> MSETQSQTMTRPQDLSLSDINSTVEVPEGHSFWKTLLAYSGPGALVAVGYMDPGNWSTSITGGQNFQYLLLSIIVISSLLAMLLQNMAAKLGIVCQLDLAQAIRARTSRRLGFIFWILTELAIMATDIAAVIGAAIALYLLFKIPIFLAVVITVLDVFLLLLLNRIGFRKIEALVVCLIFVILFVFLYQIILSQPAWHQVAKGLIPSWASVQTSPKIGGQTPLSASLGIIGATIMPHNLFLHSAISQSRKIDRTDSSKVAEAVRFSNWDSNIQLSLAMVVNALLLIMGVAVFKSGAVQDPSFFGLYQALSNPDMVSNPVLAEAARSGVLSTLFAVALLASGQNSTITGTITGQVIMEGFIHLRLPLWLRRLVTRLIAIIPVVVCVAITSHQGSLDEHQALNNLMNNSQVFLALALPFSIVPLLMLTDSAAQMGNQFKNTRWVKVMGWLTVIILTLLNLISISSQIAGFFGDNPSSQDLLLSQVISIGIILAMIGLLIWTIIDIRRFTHPKQKALEVLFQ

conserved and function as secondary active transporters. transport proteins that include the amino acid transporter LeuT18. μM range and that metal ion transport is coupled to the cotransport of protons. of the prokaryotic SLC11 transporter EcoDMT.

mutants of Glu129 and reduced to half in H236A. different role in proton-coupled metal ion transport. does not function as primary H+-acceptor. the pKa of Glu129 would have to be shifted upwards. in vicinity to the metal ion coordinating Asp51.>[2x]HHHHHHIEGRGAYVLDDSDGLGREFDGIGAVSGGGATSRLLVNYPEPYRSEILDYLFKPNFGASLHILKVEIGGDGQTTDGTEPSHMHYELDENYFRGYEWWLMKEAKKRNPDIILMGLPWSFPGWLGKGFSWPYVNLQLTAYYVVRWILGAKHYHDLDIDYIGIWNERPFDANYIKELRKMLDYQGLQRVRIIASDNLWEPISSSLLLDQELWKVVDVIGAHYPGTYTVWNAKMSGKKLWSSEDFSTINSNVGAGCWSRILNQNYINGNMTSTIAWNLVASYYEELPYGRSGLMTAQEPWSGHYVVASPIWVSAHTTQFTQPGWYYLKTVGHLEKGGSYVALTDGLGNLTIIIETMSHQHSMCIRPYLPYYNVSHQLATFTLKGSLREIQELQVWYTKLGTPQQRLHFKQLDTLWLLDGSGSFTLELEEDEIFTLTTLTTGRKGSYPPPPSSKPFPTNYKDDFNVEYPLFSEAPNFADQTGVFEYYMNNEDREHRFTLRQVLNQRPITWAADASSTISVIGDHHWTNMTVQCDVYIETPRSGGVFIAGRVNKGGILIRSATGVFFWIFANGSYRVTADLGGWITYASGHADVTAKRWYTLTLGIKGYFAFGMLNGTILWKNVRVKYPGHGWAAIGTHTFEFAQFDNFRVEAAR;>MGKSLPCDICKTVVTEAGNLLKDNATQEEILHYLEKTCEWIHDSSLSASCKEVVDSYLPVILDMIKGEMSNPGEVCSALNLCQSLQE[2x]

For example, Krabbe disease is caused by loss of galactocerebrosidase (GALC) which is responsible for the removal of the terminal galactose from the glycosphingolipid galactocerebroside (GalCer). Importantly, mutation of the GALC-associated saposin SapA can also cause Krabbe disease. To remedy this deficit we have solved the structure of GALC in complex with SapA, defining how saposins solubilise lipids for processing by soluble hydrolases. Here we reveal molecular details of how glycosphingolipids can be bound by SapA and presented to the active site of GALC for catabolic processing.

Based on these insights, the GALC–SapA complex was formed at pH 5.0 in the presence of the detergent LDAO and the X-ray crystal structure of this complex solved and refined to 3.6 Å resolution. The structure reveals that the complex forms a 2:2 heterotetramer, composed of a central SapA dimer with two molecules of GALC binding its surface. Importantly, the active site of GALC is buried in the centre of the interaction interface. At the optimal pH of the interaction the GALC and SapA surfaces demonstrate extensive charge complementarity, explaining the observed pH dependency of the interaction. Analysis of the SapA dimer in the complex structure suggests the presence of disordered detergent within the core. A cross-section through the structure at this position shows that this hydrophobic patch encircles an opening in the SapA dimer surface that lies directly opposite the GALC active site. This reveals a continuous open channel that stretches from the GALC active site through to the hydrophobic cavity buried in the SapA dimer. The hydrophobic acyl chains of glycosphingolipids such as GalCer can thus be shielded from the polar solvent by the SapA dimer, while the hydrophilic glycosyl head groups are presented to the GALC active site. In our structure the monomers are head-to-head, with all termini together at one end, while in the published lipoprotein disc structure the monomers adopt a head-to-tail orientation.> AQLRQFYVAAQGISWSYRPEPTNSSLNLSVTSFKKIVYREYEPYFKKEKPQSTISGLLGPTLYAEVGDIIKVHFKNKADKPLSIHPQGIRYSKLSEGASYLDHTFPAEKMDDAVAPGREYTYEWSISEDSGPTHDDPPCLTHIYYSHENLIEDFNSGLIGPLLICKKGTLTEGGTQKTFDKQIVLLFAVFDESKSWSQSSSLMYTVNGYVNGTMPDITVCAHDHISWHLLGMSSGPELFSIHFNGQVLEQNHHKVSAITLVSATSTTANMTVGPEGKWIISSLTPKHLQAGMQAYIDIKNCPKKTRNLKKITREQRRHMKRWEYFIAAEEVIWDYAPVIPANMDKKYRSQHLDNFSNQIGKHYKKVMYTQYEDESFTKHTVNPNMKEDGILGPIIRAQVRDTLKIVFKNMASRPYSIYPHGVTFSPYEDEVNSSFTSGRNNTMIRAVQPGETYTYKWNILEFDEPTENDAQCLTRPYYSDVDIMRDIASGLIGLLLICKSRSLDRRGIQRAADIEQQAVFAVFDENKSWYLEDNINKFCENPDEVKRDDPKFYESNIMSTINGYVPESITTLGFCFDDTVQWHFCSVGTQNEILTIHFTGHSFIYGKRHEDTLTLFPMRGESVTVTMDNVGTWMLTSMNSSPRSKKLRLKFRDVKCIPDDDEDSYEIFEPPESTVMATRKMHDRLEPEDEESDADYDYQNRLAAALGIR;> SNN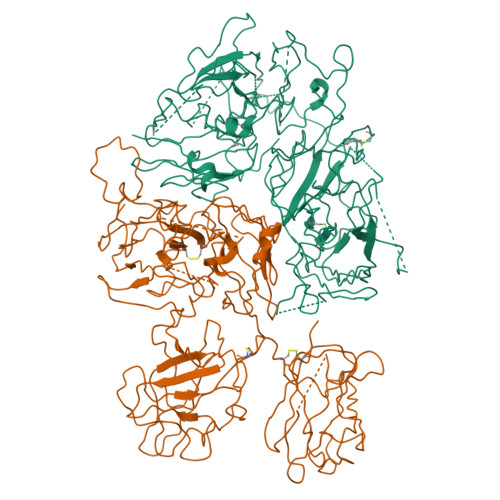GNRRNYYIAAEEISWDYSEFVQRETDIEDSDDIPEDTTYKKVVFRKYLDSTFTKRDPRGEYEEHLGILGPIIRAEVDDVIQVRFKNLASRPYSLHAHGLSYEKSSEGKTYEDDSPEWFKEDNAVQPNSSYTYVWHATERSGPESPGSACRAWAYYSAVNPEKDIHSGLIGPLLICQKGILHKDSNMPMDMREFVLLFMTFDEKKSWYYEKKSRSSWRLTSSEMKKSHEFHAINGMIYSLPGLKMYEQEWVRLHLLNIGGSQDIHVVHFHGQTLLENGNKQHQLGVWPLLPGSFKTLEMKASKPGWWLLNTEVGENQRAGMQTPFLIMDRDCRMPMGLSTGIISDSQIKASEFLGYWEPRLARLNNGGSYNAWSVEKLAAEFASKPWIQVDMQKEVIITGIQTQGAKHYLKSCYTTEFYVAYSSNQINWQIFKGNSTRNVMYFNGNSDASTIKENQFDPPIVARYIRISPTRAYNRPTLRLELQGCEVNGCSTPLGMENGKIENKQITASSFKKSWWGDYWEPFRARLNAQGRVNAWQAKANNNKQWLEIDLLKIKKITAIITQGCKSLSSEMYVKSYTIHYSEQGVEWKPYRLKSSMVDKIFEGNTNTKGHVKNFFNPPIISRFIRVIPKTWNQSIALRLELFGCDIY>YEEEDVICDGCNGPVVGTRYKCSVCPDYDLCSVCEGKGLHRGHTKLAFPSPFGHLSEGFS[4x]

Intriguingly, the autophagy adapter p62/SQSTM1/Sequestosome-1 was recently reported to recognize N-degrons, the N-end rule substrates of the well-characterized UPS, and where ultimately these substrates are delivered to ALS8,9. p62 is a key selective autophagy adapter that plays a role in the degradation of various cellular constituents such as misfolded proteins and their aggregates, malfunctioning organelles, and invading pathogens. Intriguingly, it was recently reported that the central ZZ-domain in p62 plays a critical role in the recognition of N-terminal arginylated BiP/GRP78 by the Arg-tRNA transferase ATE1. Here, we present the high resolution structures of the ZZ-domain of p62 in complex with 8 different N-degrons including type-1 and type-2, and subsequently identify key determinants involved in the unusual recognition.

However, a recent report has shown that the ZZ-domain of p62 also recognizes type-2 N-degrons, although with weaker affinity than with type-1 N-degrons. Therefore, we determined the structure of the ZZ-domain in complex with a variety of N-degrons comprising three type-1 N-degrons and five type-2 N-degrons. As described for the R-BiP complex, two aspartic acid residues, Asp129 and Asp149, bind to the α-amino group, and Asp147 forms a hydrogen bond with the first peptide bond, which means that these interactions are conserved in all different N-terminal residues. However, the side chain of the N-terminal residue of the N-degron is recognized differently. The side chain of Asn132 which undergoes a conformational change plays a critical role in interacting with the first residue of the N-degron. The bipolar nature of the side chain atoms (O and N) of Asn132 allow for the recognition of positively charged type-1 substrates as well as type-2 substrates, and especially N-terminal tyrosine and tryptophan residues since they possess polar atoms in the side chain. As expected, arginine at the primary position showed the strongest binding affinity with, intriguingly, tyrosine and tryptophan residues following in second and third place, respectively. Our structural and biochemical measurement data showed that the presence of tyrosine or tryptophan at the primary position resulted in relatively high affinity because these side chains contain polar atoms, oxygen in tyrosine and nitrogen in tryptophan that can form hydrogen bonds with the side chain of Asn132 of the ZZ-domain. Our structural information clearly explains the affinity measurement data as well as previous pull-down assay results showing that type-1 N-degrons and only a subset of type-2 N-degron peptides (Phe, Trp, and Tyr) displayed binding affinity with p62.> SNAMSNVLIINAMKEFAHSKGALNLTLTNVAADFLRESGHQVKITTVDQGYDIESEIENYLWADTIIYQMPAWWMGEPWILKKYIDEVFTDGHGRLYQSDGRTRSDATKGYGSGGLIQGKTYMLSVTWNAPREAFTDPEQFFHGVGVD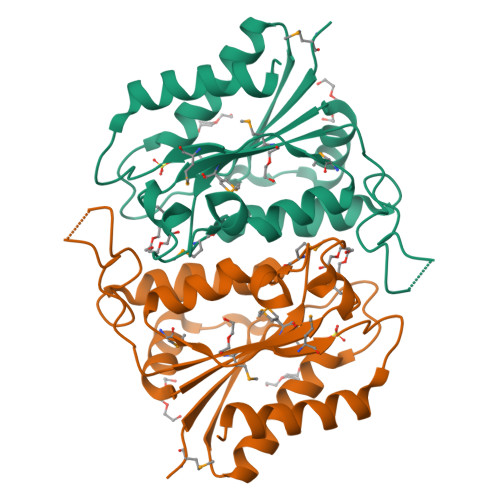GVYLPFHKANQFLGMKPLPTFMCNDVIKQPDIEGDIARYRQHLAENVNS> NLFQFARMINGKLGAFSVWNYISYGCYCGWGGQGTPKDATDRCCFVHD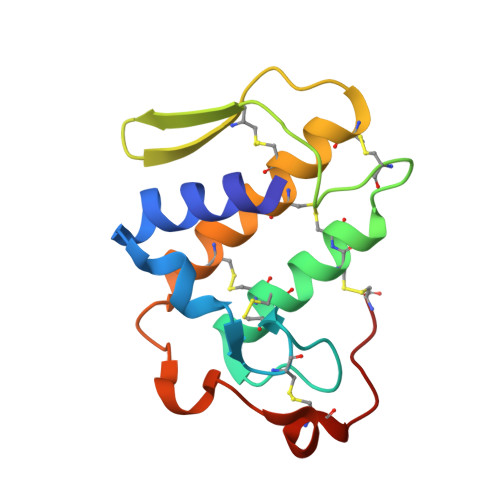CCYGGVKGCNPKLAIYSYSFQRGNIVCGRNNGCLRTICECDRVAANCFHQNKNTYNKEYKFLSSSKCRQRSEQC> MHHHHHHGSACFAKGTNVLMADGSIECIENIEVGNKVMGKDGRPREVIKLPRGSETMYSVVQKSQHRAHKSDSSREMPELLKFTCNATHELVVRTPRSVRRLSRTIKGVEYFEVITFEMGQKKAPDGRIVELVKEVSKSYPVSEGPERANELVESYRKASNKAYFEWTI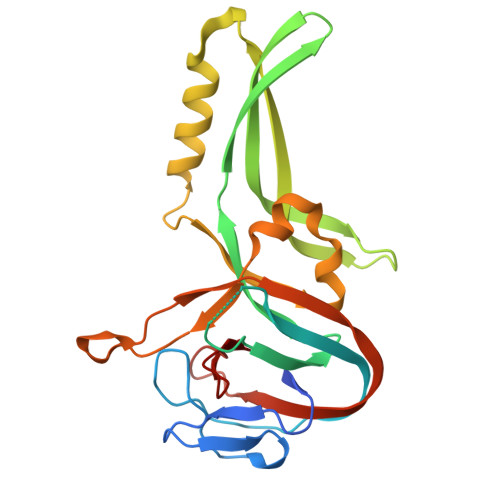EARDLSLLGSHVRKATYQTYAPIGAAFARECRGFYFELQELKEDDYYGITLSDDSDHQFLLANQVVVH> UUACUGUGAGAAUCAGUAACAAACAUGUGGGGCUUAUAUCUAAUCUUCGGAUU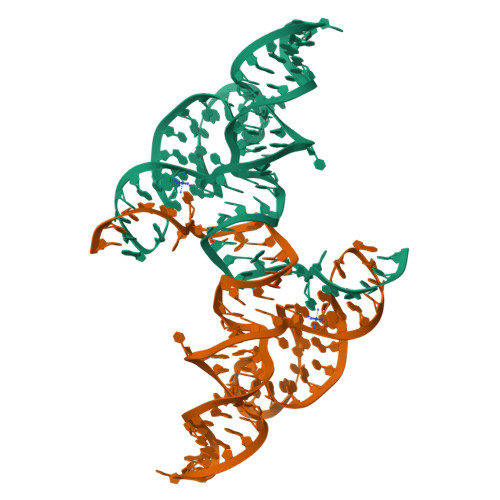AGUAUUAGUGCAGACGUUAAAACCAUGU>EYGYIVTDQKPLSL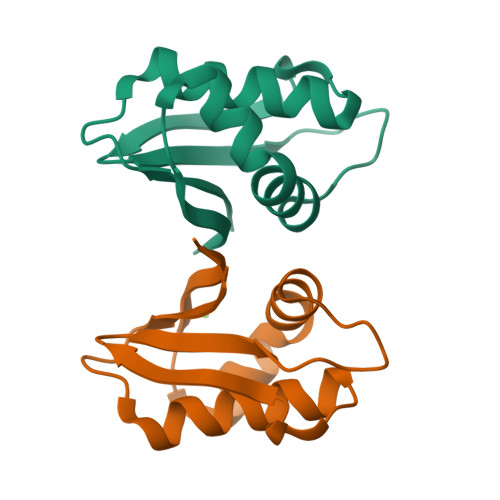AAGVKLLEILAEHVHMSSGSFINIAVVGPALTFRIRHNEQNLSLADVTQQAGLVKSELEAQTGLQILQTGVGQRE[2x]>GP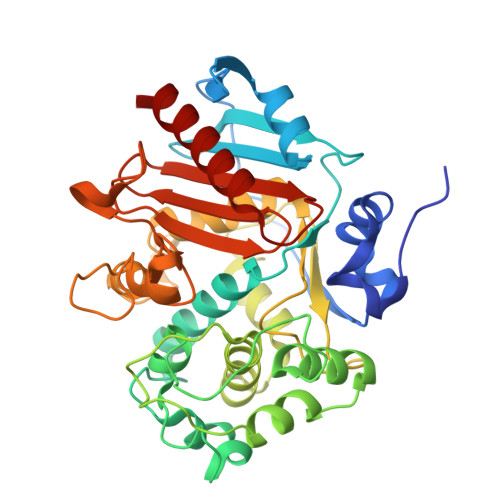DAAVENPRIGRAADLYELIPEYQPDTYRNMDKVYPTRVIHKGTKVRPLPAGVAIAPRYRIGGEEYGVDDFMRRNRVGGVLVLKDGKVALERYGLGNDERTRWTSFSVVKSISSTLVGAAVQQGLLALDQPVDKYLPSLAGSAYQGVTVEQVLQMSSGVRWNETYRDPKSDRRQMFDAQLAERPGGILRLLASLPRQYPSGTHFTYSTGESHLQSELLHAATRIPVSDYLSERIWARMGMESDGFWQLESPAGQEIGSSGLSATLRDYGRFGQFVLEDGVIDGERILPEGWVDRASRVEASSHLAPGKLYDGEYALGYGYQWWTFPVGAKALPEHDGGAFEAQGIFGQYLYINRKEKIVAVVWSAWPKPEMDDREEETYAFLGAAVKALR[4x]>[4x]DTEMEEVD;>EEWLDILGNGL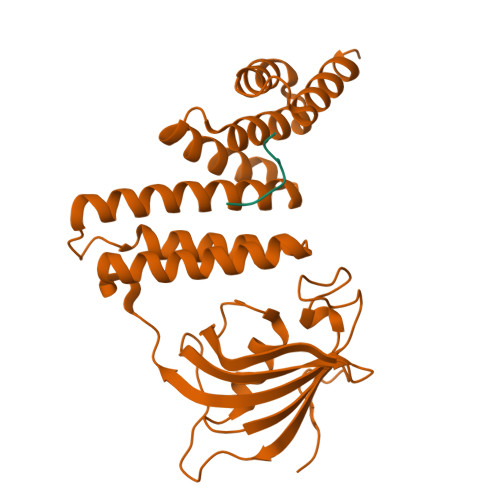LRKKTLVPGPPGSSRPVKGQVVTVHLQTSLENGTRVQEEPELVFTLGDCDVIQALDLSVPLMDVGETAMVTADSKYCYGPQGRSPYIPPHAALCLEVTLKTAVDGPDLEMLTGQERVALANRKRECGNAHYQRADFVLAANSYDLAIKAITSSAKVDMTFEEEAQLLQLKVKCLNNLAASQLKLDHYRAALRSCSLVLEHQPDNIKALFRKGKVLAQQGEYSEAIPILRAALKLEPSNKTIHAELSKLVKKHAAQRSTETALYRKMLGNPSRLPAKCPG[4x]>MDRPQERMVGELRDLSPDDPQVQKAAQA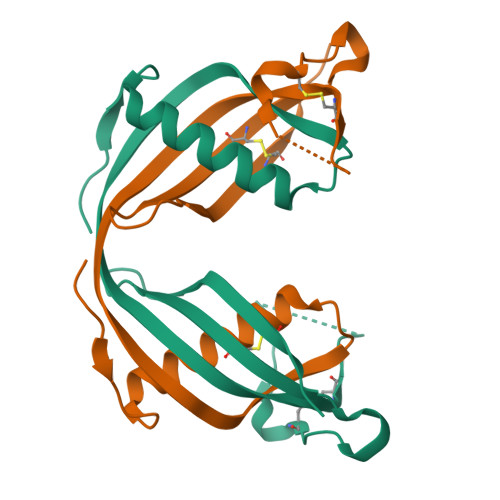AVASYNMGSNSIYYFRDTHIIKAQSQLVAGIKYFLTMEMGSTDCRKTRVTGDHVDLTTCPLAAGAQQEKLRCDFEVLVVPWQNSSQLLKHNCVQMLEHHHHHH[2x]>MMEFTIKRDYFITQLNDTLKAISPRTTLPILTGIKIDAKEHEVILTGSDSEISIEITIPKTVDGEDIVNISETGSVVLPGRFFVDIIKKLPGKDVKLSTNEQFQTLITSGHSEFNLSGLDPDQYPLLPQVSRDDAIQLSVKVLKNVIAQTNFAVSTSETRPVLTGVNWLIQENELICTATDSHRLAVRKLQLEDVSENKNVIIPGKALAELNKIMSDNEEDIDIFFASNQVLFKVGNVNFISRLLEGHYPDTTRLFPENYEIKLSIDNGEFYHAIDRASLLAREGGNNVIKLSTGDDVVELSSTSPEIGTVKEEVDANDVEGGSLKISFNSKYMMDALKAIDNDEVEVEFFGTMKPFILKPKGDDSVTQLILPIRTY[2x];>MLFFKEKFY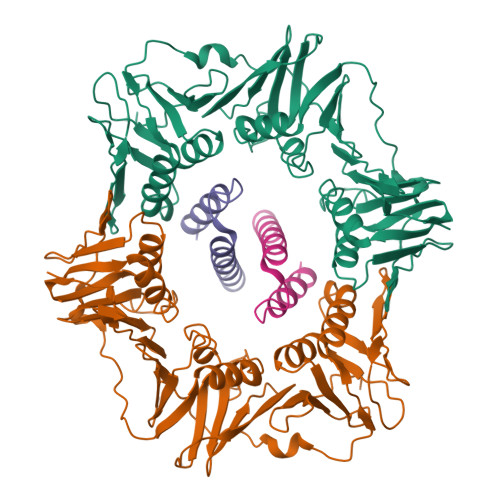NELSYYRGGHKDLESMFELALEYIEKLEEEDEQQVTDYENAMEEELRDAVDVIESQLEIIKDIVR[2x]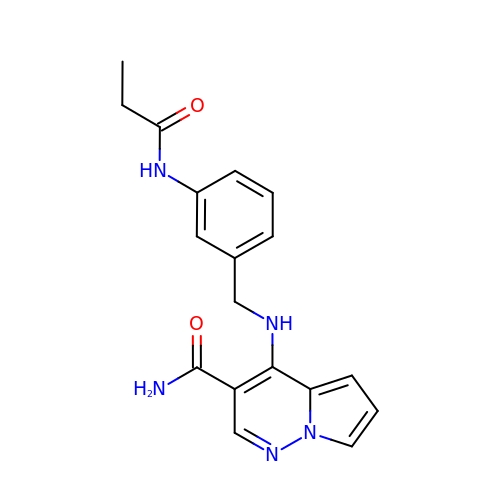4-({[3-(propanoylamino)phenyl]methyl}amino)pyrrolo[1,2-b]pyridazine-3-carboxamide | C18 H19 N5 O2 | NLMYDZAEGAXRHW-UHFFFAOYSA-N>[2x]MSPTAFPAAETATAPATAVDPGPELDGGDFALPEGGLDDDRRLRALDAVDEYLTRKRKHLVGYAATQDMQGTALDLARFMPNNINNLGDPFQSGGYKPNTKVVERAVLDYYAKLWHAERPHDPADPESYWGYMLSMGSTEGNMYALWNARDYLSGKALIQPPTAPFDAVRYVKADPDRRNPNAHHPVAFYSEDTHYSFAKAVAVLGVETFHAVGLEKYADECPLVDPVTGLRTWPTEVPSRPGPSGLSWDGPGEIDVDALAVLVEFFAAKGHPVFVNLNLGSTFKGAHDDVRAVCERLLPIFERHGLVQREVVYGSCPQTGRPLVDVRRGFWIHVDGALGAGYAPFLRLAAEDPEGYGWTPEAELPEFDFGLRLPTAGHGEVDMVSSIAMSGHK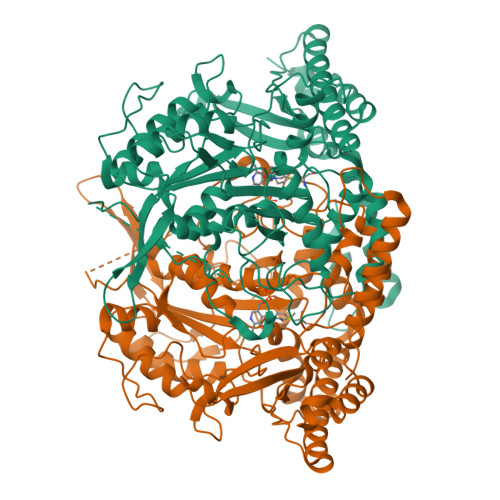WAGAPWPCGIYMTKVKYQISPPSQPDYIGAPDTTFAGSRNGFSPLILWDHLSRYSYRDQVERIREAQELAAYLERRLTAMERELGVELWPARTPGAVTVRFRKPSAELVAKWSLSSQDVLMVPGDETTRRSYVHVFVMPSVDRAKLDALLAELAEDPVILGAP> GPGSMGSVQRQDLVLFSDQSVLPAHFFQDSNSHNLFFITHQSCTQPLWMINALVETHVLGSPSSLNESSSSMLPSSTRSHAVLASFIHEQNYFTNSLNKLKIPSNNYNVLDFLSDFIVNNIHNKPRDKILSDVLAKFSAAIQNNPTDTIVIIEQPELLLSLVSGLTCSELNNKFITPLLRQCKVLIIVSNSDIFNIDEYDASVHSSNLQNFYKSSFIKSMINLNLNPLKTGF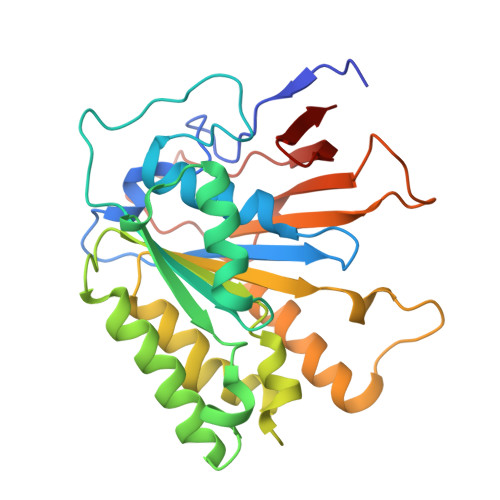AKDVTGSLHVCRGGAPIATSNTSLHVVENEYLYLNEKESTKLFYR>MIPVTELRYFADTQPAYRILKPWWDVFTDYISIVMLMIAVFGGTLQVTQDKMICLPCKWVTKDSCNDSFRGWAASSPEPTYPNSTVLPTPDTGPTGIKYDLDRHQYNYVDAVCYENRLHWFAKYFPYLVLLHTLIFLACSNFWFKFPRTSSKLEHFVSILLKCFDSPWTTRALSETVVEESDPKPAFSKMNGSMDKKSSTVSEDVEATVPMLQRTKSRIEQGIVDRSETGVLDKKEGEQAKALFEKVKKFRTHVEEGDIVYRLYMRQTIIKVIKFALIICYTVYYVHNIKFDVDCTVDIESLTGYRTYRCAHPLATLFKILASFYISLVIFYGLICMYTLWWMLRRSLKKYSFESIREESSYSDIPDVKNDFAFMLHLIDQYDPLYSKRFAVFLSEVSENKLRQLNLNNEWTLDKLRQRLTKNAQDKLELHLFMLSGIPDTVFDLVELEVLKLELIPDVTIPPSIAQLTGLKELWLYHTAAKIEAPALAFLRENLRALHIKFTDIKEIPLWIYSLKTLEELHLTGNLSAENNRYIVIDGLRELKRLKVLRLKSNLSKLPQVVTDVGVHLQKLSINNEGTKLIVLNSLKKMVNLTELELIRCDLERIPHSIFSLHNLQEIDLKDNNLKTIEEIISFQHLHRLTCLKLWYNHIAYIPIQIGNLTNLERLYLNRNKIEKIPTQLFYCRKLRYLDLSHNNLTFLPADIGLLQNLQNLAVTANRIEALPPELFQCRKLRALHLGNNVLQSLPSRVGELTNLTQIELRGNRLECLPVELGECPLLKRSGLVVEEDLFSTLPPEVKERLWRADKEQASNSLEVLFQG[6x]

The underlying channels, termed volume-regulated anion channels (VRACs) have variable selectivity and conductance between cells, but are similarly activated by osmotic stimuli and blocked by small molecule anionic inhibitors including DCPIB (4-[(2-Butyl-6,7-dichloro-2-cyclopentyl-2,3-dihydro-1-oxo-1H-inden-5-yl)oxy]butanoic acid). LRRC8A forms a 565 kDa, homohexameric channel with each monomer consisting of (from extracellular to intracellular side) an extracellular cap, four transmembrane spanning helices TM1-4, a linker region, and a LRR domain. Here, we report structures of the homohexameric LRRC8A channel embedded in lipid nanodiscs in the presence and absence of the inhibitor DCPIB determined by cryo-electron microscopy. The N-terminal arginine residue of this helix (R103) projects in towards the conduction axis to form the highly electropositive selectivity filter of the anion-selective channel.

To this end, LRRC8A was solubilized and purified in detergent, exchanged into lipid nanodiscs formed by the membrane scaffold protein MSP1E3D1 and phosphatidylcholine lipids (POPC, 1-palmitoyl-2-oleoyl-sn-glycero-3-phosphocholine), and vitrified in the presence of the LRRC8 inhibitor DCPIB. Focused classifications on the linker region indeed resolved two channel conformations: a constricted class and an expanded class. Masking out the LRRs and applying six-fold (C6) symmetry resulted in the highest resolution reconstructions: 3.21 Å resolution for the constricted and 3.32 Å resolution for the expanded class, respectively. We attribute this bi-lobed density to the DCPIB inhibitor based on size, shape, chemical considerations, and comparison to apo-LRRC8A reconstructions. The density is well fit with the predominantly hydrophobic indane, butyl, and cyclopentyl constituents in the larger lobe extracellular to the R103 ring and the negatively charged butanoic acid group in the smaller lobe adjacent to and below the guanidinium groups of the R103 ring. The structure of DCPIB bound to LRRC8A provides a simple explanation for the mechanism of drug block: DCPIB acts like a cork to plug the mouth of the channel. The R103 ring electrostatically interacts with the DCPIB carboxylic acid while the bulky hydrophobic end of the drug is too large to pass. The upper gap is filled with three well-defined tubular features that are modeled as partial POPC lipid hydrocarbon acyl chains. The presence of these ordered acyl chains seals the upper gap in the channel surface and may act as a ‘glue’ that connects adjacent subunits and stabilizes the upper transmembrane domain against movements in channel linkers and LRRs. The structure of the extracellular cap, DCPIB-bound selectivity filter, and extracellular halves of the TM region are essentially indistinguishable between the two structures (mean Cα r.m.s.d. = 0.42 Å).>[7x]NLIP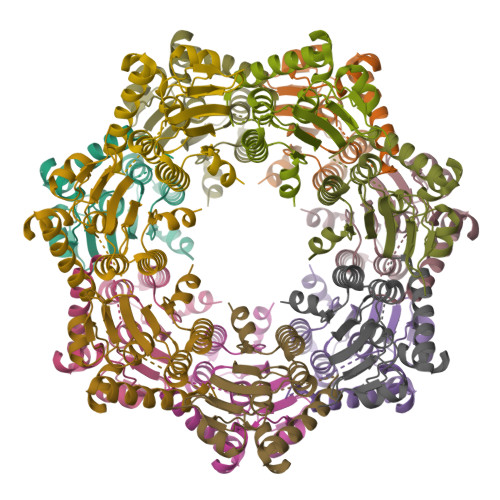TVIEQTNRGERAYDIYSRLLKDRIIMLGSAIDDNVANSIVSQLLFLAAEDPEKEISLYINSPGGSITAGMAIYDTMQFIKPKVSTICIGMAASMGAFLLAAGEKGKRYALPNSEVMIHQPLGGAQGQATEIEIAAKRILLLRDKLNKVLAERTGQPLEVIERDTDRDNFKSAEEALEYGLIDKILTHTEDKK> MRRNIFCLACLWIVQACLSLDRADILYNIRQTSRPDVIPTQ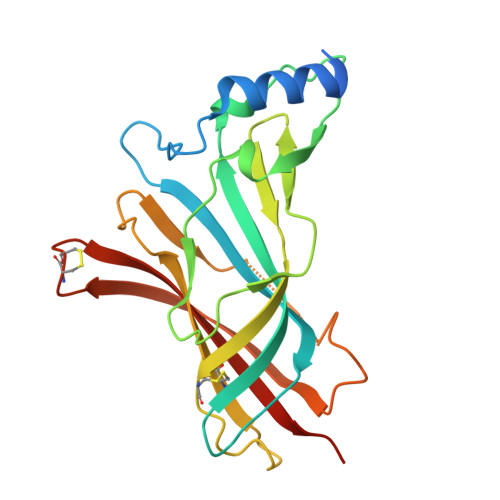RDRPVAVSVSLKFINILEVNEITNEVDVVFWQQTTWSDRTLAWNSSHSPDQVSVPISSLWVPDLAAYNAISKPEVLTPQLAHVVSDGEVQYTPSIRQRFSCDVSGVDTQSGATCRIKIGSWTHHSREISVDPTTENSDDSEYFSQYSRFEILDVTQKKNSVTYSCCPEAYEDVEVSLNFRKKGRSEIL>[6x]MTEPLPRIQHYEDLGLGLFIHWGLYSQMAVGEWTELIHHRNQHDYEQLIKTFTAAQFDAKKIAHAAKAVGAKYIVLTTKHHEGFFLYDTKGLSDFDVMHAPARRDLIAEFVAACREEDLLPFFYMATYDWHTPLYDDDFPAYLTYLQKSVEVLCRNYGPVGGFWFDGNWNKKDADWHLPELYGMIRHYQPNAIIVSN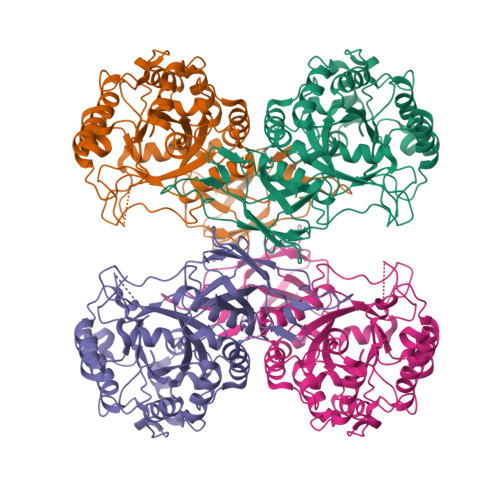TGLKNRGQVSDPEIDVVTYERRTPDEIYHGAPNEKYVAGEISITLNQHWGIAANDLNYKSPAEMIETVAHARHIGANILVNIGLTGTGAIPAAAQTYMHLLGRWTAMAAPVLYKGRPVPVTSAHGTRDFVLHTSKHDFLCILDLQVVGKDNVVLGGEGVNPRSFVGIGQPIQRIHWLDNDEVLSFTQDLDKKVLTVDATGYPYGSDWVVRIAQIDYE> ETGDVKPDLQTKQDKVLAHFIGNSTDYFKILDHNDEFVLVGAKDVIYNVSLNGLKEIARLEWHSTDADRELCALKGKHEWDCHNYLRVYALRPNGEVLLCGTNSYKPRCRHYTPVEVSSEEAGSAGHAHAMRYEVSRDVEAQGLCPYSPAHNSTYAFADGHLYSATVADFSGGDPLIYRENLRTEQYDLKQLNQPDFVGAIERNGYVLFFFRELSMEVMNFGKAVYSRVARVCKNDRGGPYSHGKSWTSFLKARLNCSVPGEFPFYFDEIQAISPIVESGSKSLIYAVFTTSVNAIPGSAVCAFNVDDILAAFDGEFKSQKDSQSHWLPVEREQVPKPRPGQCVEDSRTLTSIAVNFIKNHPLMEEAVPAVHGRPLLTKVNLHHRLTAIAVHPQVKSLSGAYYDVIYSGTDDGKVTKFINILS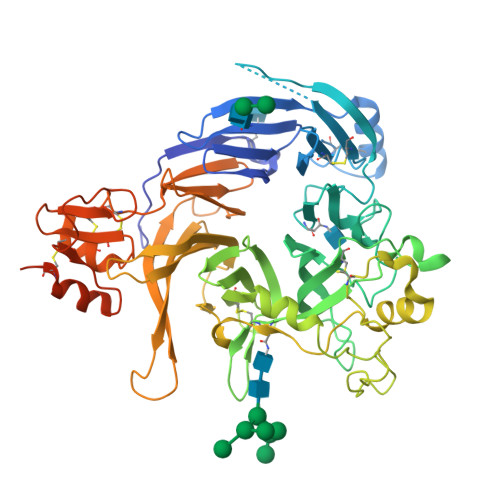THPNSTVDRLKTVVISEMQVLPLGTPIRELVISTSKNSLVVVSDGSLVSVPLHHCSHIVDCLGCLSLQDPICAWDLQTHECKNLATSQHKFGTKTYLQSLNSTKKAAALLCPHIPRDAPGAETVSFVTMAPPPTEEQKLLYSNVGSGTKHHHHHH The origin recognition complex (ORC), composed of Orc1–6, is a highly conserved heterohexameric complex, which plays a critical role in recognizing origin DNA and promoting helicase loading. Each of the Orc1–5 subunits bears an AAA+ or AAA+-like domain and an α-helical winged-helix domain (WHD). Among Orc1–5, Orc1, Orc4, and Orc5 each contains a functional AAA+ domain for nucleotide binding; in contrast, Orc2 and Orc3 only contain a RecA-like subdomain with no predicted ATPase activities. Away from DNA, metazoan ORC resides in an autoinhibited conformation with a closed and constricted central channel to preclude DNA binding.

ORC1 and ORC6 co-purified with ORC2 were in much lower amount when compared with other ORC subunits. With these general similarities, however, ORC2-WHD displays a very different conformation from all previously reported structures. The most significant contribution to this interface appears to be from the helix-turn-helix (HTH) motif (α3 and α4) of ORC2-WHD. The loop region of this HTH is positioned very close to the cleft between AAA+ domains of ORC4 and ORC5 with its Phe524 docked into a hydrophobic pocket formed by the residues from ORC4-RecA (Ile105, Leu163, His166) and ORC5-RecA (Ala135, Asn136). In addition, Arg521 and Asn527 of ORC2 form hydrogen bonds with Asp132 and Glu134 of ORC5, respectively. Moreover, most of the DNA binding motifs of ORC subunits, such as the initiation-specific motif (ISM) from RecA subdomain and the β-hairpin motif from WHD, are blocked by these interactions. In contrast, although DmORC structure also assumes an autoinhibited conformation, its central channel is not fully occupied by ORC2-WHD, leaving a hollow ring with a diameter of 10–14 Å.

> MSKPELKEDKMLEVHFVGDDDVLNHILDREGGAKLKKERAQLLVNPKKIIKKPEYDLEEDDQEVLKDQNYVEIMGRDVQESLKNGSATGGGNKVYSFQNRKHSEKMAKLASELAKTPQKSVSFSLKNDPEITINVPQSSKGHSASDKVQPKNNDKSEFLSTAPRSLRKRLIVPRSHSDSESEYSASNSEDDEGVAQEHEEDTNAVIFSQKIQAQNRVVSAPVGKETPSKRMKRDKTSDLVEEYFEAHSSSKVLTSDRTLQKLKRAKLDQQTLRNLLSKVSPSFSAELKQLNQQYEKLFHKWMLQLHLGFNIVLYGLGSKRDLLERFRTTMLQDSIHVVINGFFPGISVKSVLNSITEEVLDHMGTFRSILDQLDWIVNKFKEDSSLELFLLIHNLDSQMLRGEKSQQIIGQLSSLHNIYLIASIDHLNAPLMWDHAKQSLFNWLWYETTTYSPYTEETSYENSLLVKQSGSLPLSSLTHVLRSLTPNARGIFRLLIKYQLDNQDNPSYIGLSFQDFYQQCREAFLVNSDLTLRAQLTEFRDHKLIRTKKGTDGVEYLLIPVDNGTLTDFLEKEEEEA;> MATSSMSKGCFVFKPNSKKRKISLPIEDYFNKGKNEPEDSKLRFETYQLIWQQMKSENERLQEELNKNLFDNLIEFLQKSHSGFQKNSRDLGGQIKLREIPTAALVLGVNVTDHDLTFGSLTEALQNNVTPYVVSLQAKDCPDMKHFLQKLISQLMDCCVDIKSKEEESVHVTQRKTHYSMDSLSSWYMTVTQKTDPKMLSKKRTTSSQWQSPPVVVILKDMESFATKVLQDFIIISSQHLHEFPLILIFGIATSPIIIHRLLPHAVSSLLCIELFQSLSCKEHLTTVLDKLLLTTQFPFKINEKVLQVLTNIFLYHDFSVQNFIKGLQLSLLEHFYSQPLSVLCCNLPEAKRRINFLSNNQCENIRRLPSFRRYVEKQASEKQVALLTNERYLKEETQLLLENLHVYHMNYFLVLRCLHKFTSSLPKYPLGRQIRELYCTCLEKNIWDSEEYASVLQLLRMLAKDELMTILEKCFKVFKSYCENHLGSTAKRIEEFLAQFQSLDETKEEEDASGSQPKGLQKTDLYHLQKSLLEMKELRRSKKQTKFEVLRENVVNFIDCLVREYLLPPETQPLHEVVYFSAAHALREHLNAAPRIALHTALNNPYYYLKNEALKSEEGCIPNIAPDICIAYKLHLECSRLINLVDWSEAFATVVTAAEKMDANSATSEEMNEIIHARFIRAVSELELLGFIKPTKQKTDHVARLTWGGC;> MSSRKSKSNSLIHTECLSQVQRILRERFCRQSPHSNLFGVQVQYKHLSELLKRTALHGESNSVLIIGPRGSGKTMLINHALKELMEIEEVSENVLQVHLNGLLQINDKIALKEITRQLNLENVVGDKVFGSFAENLSFLLEALKKGDRTSSCPVIFILDEFDLFAHHKNQTLLYNLFDISQSAQTPIAVIGLTCRLDILELLEKRVKSRFSHRQIHLMNSFGFPQYVKIFKEQLSLPAEFPDKVFAEKWNENVQYLSEDRSVQEVLQKHFNISKNLRSLHMLLMLALNRVTASHPFMTAVDLMEASQLCSMDSKANIVHGLSVLEICLIIAMKHLNDIYEEEPFNFQMVYNEFQKFVQRKAHSVYNFEKPVVMKAFEHLQQLELIKPMERTSGNSEREYQLMKLLLDNTQIMNALQKYPNCPTDVRQWATSSLSWL;> MPHLENVVLCRESQVSILQSLFGERHHFSFPSIFIYGHTASGKTYVTQTLLKTLELPHVFVNCVECFTLRLLLEQILNKLNHLSSSEDGCSTEITCETFNDFVRLFKQVTTAENLKDQTVYIVLDKAEYLRDMEANLLPGFLRLQELADRNVTVLFLSEIVWEKFRPNTGCFEPFVLYFPDYSIGNLQKILSHDHPPEYSADFYAAYINILLGVFYTVCRDLKELRHLAVLNFPKYCEPVVKGEASERDTRKLWRNIEPHLKKAMQTVYLREISSSQWEKLQKDDTDPGQLKGLSAHTHVELPYYSKFILIAAYLASYNPARTDKRFFLKHHGKIKKTNFLKKHEKTSNHLLGPKPFPLDRLLAILYSIVDSRVAPTANIFSQITSLVTLQLLTLVGHDDQLDGPKYKCTVSLDFIRAIARTVNFDIIKYLYDFL>[2x]MGSSHHHHHHSSGLVPRGSHMPSYTVTVATGSQEHAGTDDYIYLSLVGSAGCSEKHLLDKGSFERGAVDSYDVTVDEELGEIQLVRIEKRKYGSNDDWYLKYITLKTPHGDYIEFPCYRW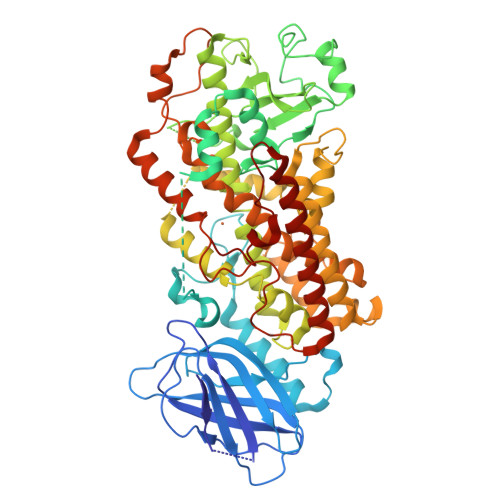ITGDVEVVLRDGRAKLARDDQIHILKQHRRKELETRQKQYRWMEWNPGFPLSIDAKCHKDLPRDIQFDSEKGVDFVLNYSKAMENLFINRFMHMFQSSWNDFADFEKIFVKISNTISERVMNHWQEDLMFGYQFLNGANPVLIRRCTELPEKLPVTTEMVECSLERQLSLEQEVQQGNIFIVDFELLDGIDANKTDPCTLQFLAAPICLLYKNLANKIVPIAIQLNQIPGDENPIFLPSDAKYDWLLAKIWVRSSDFHVHQTITHLLRTHLVSEVFGIAMYRQLPAVHPIFKLLVAHVRFTIAINTKAREQLICECGLFDKANATGGGGHVQMVQRAMKDLTYASLCFPEAIKARGMESKEDIPYYFYRDDGLLVWEAIRTFTAEVVDIYYEGDQVVEEDPELQDFVNDVYVYGMRGRKSSGFPKSVKSREQLSEYLTVVIFTASAQHAAVNFGQYDWASWIPNAPPTMRAPPPTAKGVVTIEQIVDTLPDRGRSCWHLGAVWALSQFQENELFLGMYPEEHFIEKPVKEAMARFRKNLEAIVSVIAERNENLQLPYYYLSPDRIPNSVAI> APKAKIVLVGS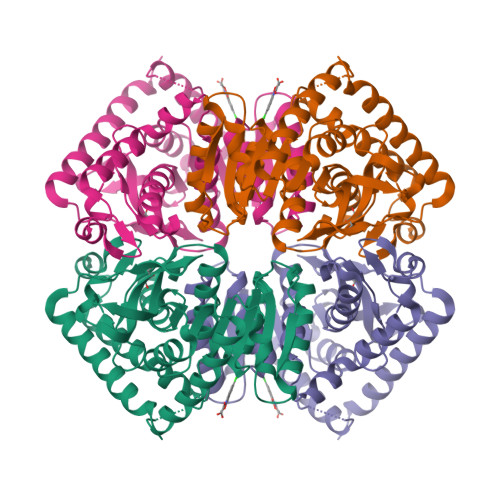GMIGGVMATLIVQKNLGDVVLFDIVKNMPHGKALDTSHTNVMAYSNCKVSGSNTYDDLAGADVVIVTAGFTKAPGKSDKEWNRDDLLPLNNKIMIEIGGHIKKNCPNAFIIVVTNPVDVMVQLLHQHSGVPKNKIIGLGGVLDTSRLKYYISQKLNVCPRDVNAHIVGAHGNKMVLLKRYITVGGIPLQEFINNKLISDAELEAIFDRTVNTALEIVNLHASPYVAPAAAIIEMAESYLKDLKKVLICSTLLEGQYGHSDIFGGTPVVLGANGVEQVIELQLNSEEKAKFDEAIAETKRMKALAHAHHHHHH>SNAMKIAIAGAGAMGSRLGIMLHQGGNDVTLIDQWPAHIEAIRKNGLIADFNGEEVVANLPIFSPEEIDHQNEQVDLIIALTKAQQLDAMFKAIQPMITEKTYVLCLLNGLGHEDVLEKYVPKENILVGITMWTAGLEGPGRVKLLGDGEIELENIDPSGKKFALEVVDVFQKAGLNPSYSSNVRYSIWRKACVNGTLNGLCTILD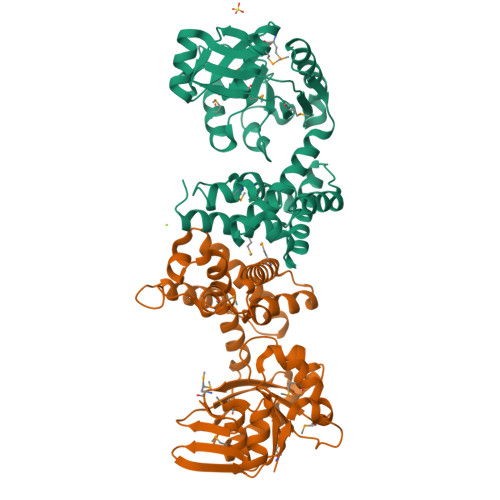CNIAEFGALPVSESLVKTLISEFAAVAEKEAIYLDQAEVYTHIVQTYDPNGIGLHYPSMYQDLIKNHRLTEIDYINGAVWRKGQKYNVATPFCAMLTQLVHGKEELLGAK[2x]> KNLDCWVDNEEDIDVILKKSTILNLDINNDIISDI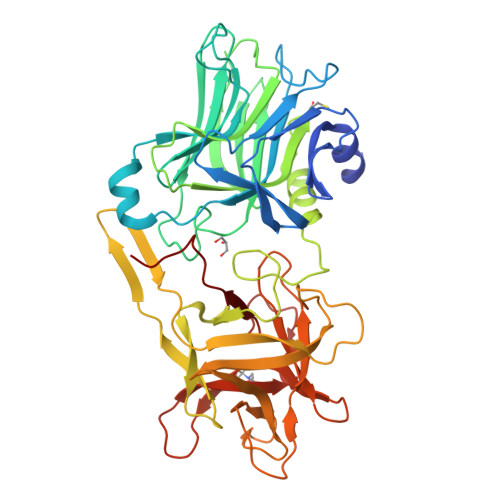SGFNSSVITYPDAQLVPGINGKAIHLVNNESSEVIVHKAMDIEYNDMFNNFTVSFWLRVPKVSASHLEQYGTNEYSIISSMKKHSLSIGSGWSVSLKGNNLIWTLKDSAGEVRQITFRDLPDKFNAYLANKWVFITITNDRLSSANLYINGVLMGSAEITGLGAIREDNNITLKLDRCNNNNQYVSIDKFRIFCKALNPKEIEKLYTSYLSITFLRDFWGNPLRYDTEYYLIPVASSSKDVQLKNITDYMYLTNAPSYTNGKLNIYYRRLYNGLKFIIKRYTPNNEIDSFVKSGDFIKLYVSYNNNEHIVGYPKDGNAFNNLDRILRVGYNAPGIPLYKKMEAVKLRDLKTYSVQLKLYDDKNASLGLVGTHNGQIGNDPNRDILIASNWYFNHLKDKILGCDWYFVPTDEGWTND(2~{S},3~{S},4~{R})-2-(hydroxymethyl)-1-(2-phenylmethoxyethyl)piperidine-3,4,5-triol | C15 H23 N O5 | 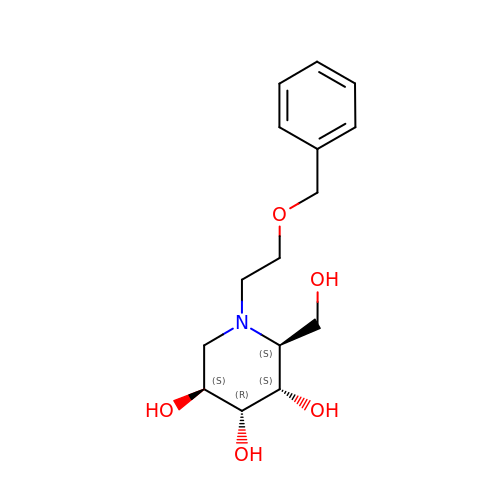IKHOHXBNNLDFIX-AVOUXACISA-N> MRRIYLNTYEQINKVKKILRKHLKNNLIGTYMFGSGVESGLKPNSDLDFLVVVSEPLTDQSKEILIQKIRPISKKIGDKSNLRYIELTIIIQQEMVPWNHPPKQEFIYGEWL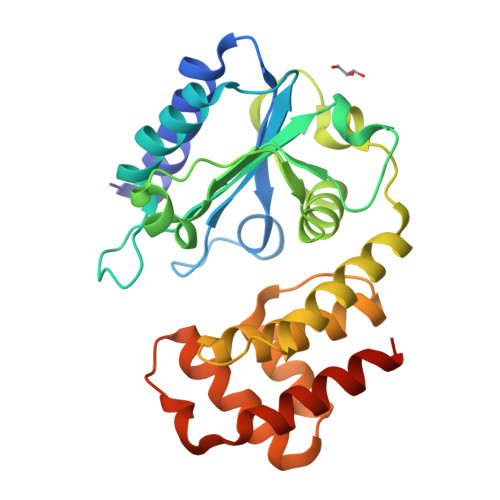QELYEQGYIPQKELNSDLTIMLYQAKRKNKRIYGNYDLEELLPDIPFSDVRRAIMDSSEELIDNYQDDETNSILTLCRMILTMDTGKIIPKDIAGNAVAESSPLEHRERILLAVRSYLGENIEWTNENVNLTINYLNNRLKKLKGHHHHHH> KFNWNKNQVIAHRGAWKKNNFPQNSIASLNE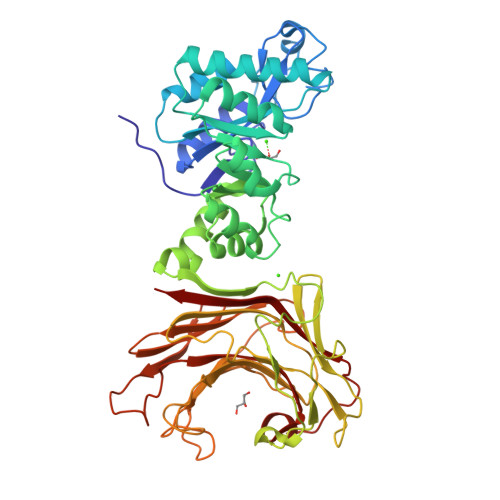AVKLGCYGSEFDVWMTADHILVVNHDPEFQGLTIEKVNYADLLTKTMSNGEKIPTLEAYLLAGKKQKSTKLILEIKPSLISKERGIEVTNKCVEMVQKLKVTDWVEYISFDYDYCKRILTLLPNAKVAYLKGEVSAEQMKADKLTGVDYHYSVYQKDNWIENAQKLGLTVNAWTVNAVPEMQWLLAHNVDYITTNEPELLFDEIKKAPVAQGWKLKWADEFDNSGLPLNKNWGYDVGGRGWGNNELQYYTDADSANAIVKKGNLNIIALKAEKENRHYTSARLVTKNKFDFKYGRVEVRAMLPKGRGLWPAIWALPTDSKYGSWPKSGEIDIMEHVGFDPDSVHGTVHTEKFNHVIHTQVGKALKVNNPYTEYHIYAIEWFTDHIDFFIDDQKYLTFKNTQKGSGDWPFDQNFHILNLAVGGNWGGKKGVDDAIFPATMKVDYVRVFQK> MSDKIIHLTDDSFDTDVLKADGAILVDFWAEWCGPSKMIAPILDEIADEY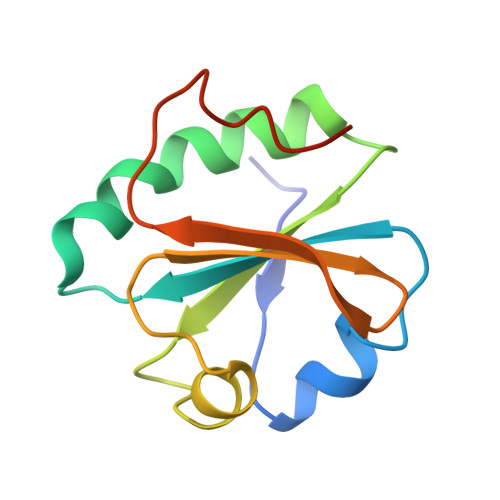QGKLTVAKLNIDQNPGTAPKYGIRGIPTLLLFKNGEVAATKVGALSKGQLKEFLDANLA>NYKKPKLLYCSNGGHFLRILPDGTVDGTRDRSDQHIQLQLSAESAGEVYIKGTETGQYLAMDTEGLLYGSQTPNEECLFLERLEENHYNTYTSKKHAEKNWFVGLKKNG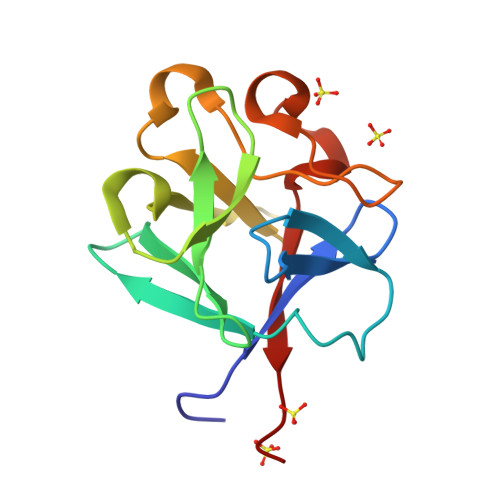SCKRGPRTHYGQKAILFLPLPVSSD[2x]O-[(S)-{[(2S)-2-(hexanoyloxy)-3-(tetradecanoyloxy)propyl]oxy}(hydroxy)phosphoryl]-D-serine | C26 H50 N 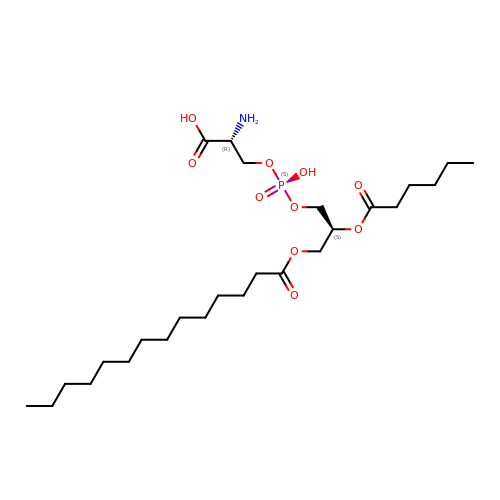O10 P | HXSPCZGHXODQMW-XZOQPEGZSA-N9-(3,4-DIHYDROXY-5-HYDROXYMETHYL-TETRAHYDRO-FURAN-2-YL)-1,9-DIHYDRO-PURINE-6-THIONE 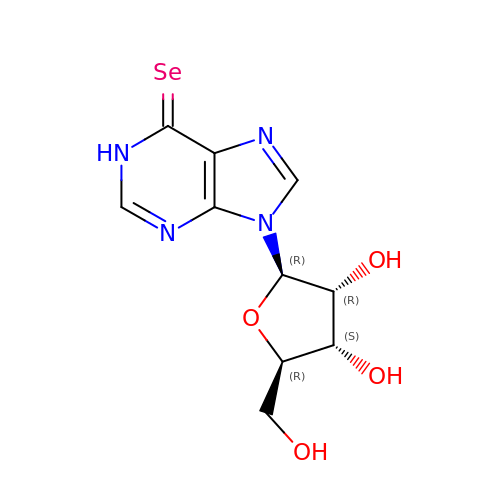| C10 H12 N4 O4 Se | MXLAAGNIPFEHEI-KQYNXXCUSA-N While some archaea produce only one type of filament, the archaeal model species Sulfolobus acidocaldarius generates four. These include rotary swimming propellers analogous to bacterial flagella (archaella), pili for twitching motility (Aap), adhesive fibres (threads), and filaments facilitating homologous recombination upon UV stress (UV pili). Here, we use cryo-electron microscopy to describe the structure of the S. acidocaldarius archaellum at 2.0 Å resolution, and update the structures of the thread and the Aap pilus at 2.7 Å and 2.6 Å resolution, respectively. We define distinct N-glycan patterns in the three filaments and identify a putative O-glycosylation site in the thread.

A deletion mutant MW039 (Δagl3), lacking the sulfoquinovose synthase Agl3 generates a trisaccharide N-glycan, missing the sulfoquinovose, one mannose and one glucose molecule. To tackle the long-standing question of how glycans impact on the architecture of motile filaments, we solved the structures of archaella and Aap and from the glycan truncation mutant Δagl3 at global resolutions of 2.4 Å and 2.6 Å, respectively, and discuss our findings in the context with previous motility experiments. Next, we purified archaella and Aap from this mutant and solved their structures by cryoEM. In the maps of the mutant archaellum and Aap, the glycans were clearly altered. The densities for the sulfoqiunovose, the terminal glucose and one mannose were missing. However, comparing the protein structures of the archaella and Aap with and without glycan truncation revealed no significant differences. These findings demonstrate that the motility-reducing effect of the glycan truncation is not due to structural changes in the archaella or Aap. Interestingly however, only the O4-linked α-mannose was missing from the N-glycan trees of the Δagl3 filaments, while the O6-linked α-mannose was still present. This suggests that the addition of the O4-linked α-mannose occurs downstream and is sensitive to the addition of sulfoquinovose. Through solving the structures of archaella and Aap from the Δagl3 mutant, we show that the structure of the filaments remains unaltered, despite the ablation of three terminal sugars, which includes the negatively charged 6-sulfoquinovose.

>LSGAIVALILVIAGVIIAIAVVLFAFGLIPGISNQGSIQVLGSGTITNSTASGSSRTIYNITITVKNTGTTSISVTSININGQPFNINGTAPSIPAGRTQPITFEVTPASGKPNFSPGASYTATIYFSNGQGAPATLIYQG[30x]>[2x]SMAHLTMPYVMPGDGEVVGVGEPVAIRFDENIADRGAAEKAIKITTNPPVEGAFYWLNNREVRWRPEHFWKPGTAVDVAVNTYGVDLGEGMFGEDNVQTHFTIGDEVIATADDNTKILTVRVNGEVVKSMPTSMGKDSTPTANGIYIV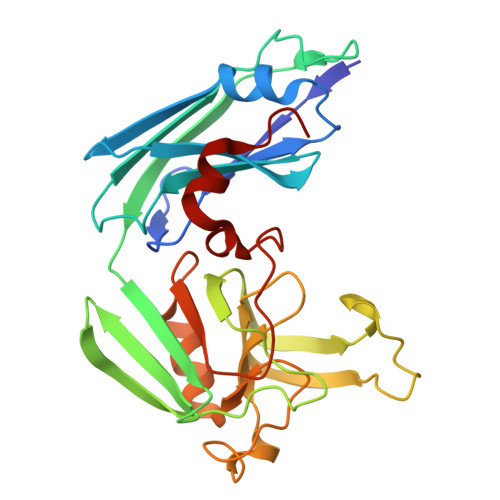GSRYKHIIMDSSTYGVPVNSPNGYRTDVDWATQISYSGVFVHSAPWSVGAQGHTNTSHGCLNVSPSNAQWFYDHVKRGDIVEVVNTVGGTLPGIDGLGDWNIPWDQWRAGNAKA> GPDRSFRWKYHQFRFLCHSNALPSHVKISVSRQTLFEDSFQQIMNMKPYDLRRRLYIIMRGEEGLDYGGIAREWFFLLSHEVLNPMYCLFEYAGKNNYCLQINPASSINPDHLTYFRFIGRFIAMALYHGKFIDTGFTLPFYKRMLNKRPTLKDLESIDPEFYNSIVWIKENNLEECGLELYFIQDMEILGKVTTHELKEGGESIRVTEENKEEYIMLLTDWRFTRGVEEQTKAFLDGFNEVAPLEWLRYFDEKELELMLCGMQEIDMSDWQKSTIYRHYTKNSKQIQWFWQVVKEMDNEKRIRLLQFVTGTCRLPVGGFAELIGSNGPQKFCIDKVGKETWLPRSHTCFNRLDLPPYKSYEQLREKLLYAIEETE;> XDPANWECRYAAFNCFIQX

Here, we report a general and rapid method for discovering α-helically constrained (Helicon) polypeptides that cooperatively induce the interaction between two target proteins without relying on previously known binders or an intrinsic affinity between the proteins. We show that Helicons are capable of binding every major class of E3 ubiquitin ligases, which are of great biological and therapeutic interest but remain largely intractable to targeting by small molecules. In addition to possessing increased stability and membrane permeability, Helicons are capable of binding large, flat protein surfaces that are inaccessible to targeting by small molecules, and Helicons have been developed to target a range of PPI targets in cells and in vivo. Characterizing Helicon-E3 co-structures and mechanisms of action, we identified new binding sites for α-helices on the E3 surfaces, as well as potential probes of the disease-linked E3, WWP123,24, highlighting the generality of our approach against this therapeutically important target class.

First, we focused on the NEDD4-like E3 ligases, which make up approximately a third of the HECT family. These include WWP1 and WWP2, which each consist of four tandem WW domains and a catalytic HECT domain at the C-terminus that transfers ubiquitin from a bound E2 first to itself and subsequently to the target substrate. Group 2 Helicons, the pan-HECT group including C73, bind both HECT domains, while Group 3 Helicons, the WWP2-HECT group including C72, bind only the WWP2 HECT domain (WWP2HECT). We next solved the crystal structures of five Helicons, four in complex with WWP2HECT representing all three groups of HECT-binding clusters, and one from Group 1 with WWP1HECT. These structures revealed three distinct Helicon binding sites on WWP2HECT. In all of the structures, we found that the HECT domains adopted similarly closed (inhibited) conformations. The WWP2 proteins in the co-structures with H301, H305, and H308 share a low root-mean-square deviation (RMSD = 0.5–0.8 Å) and are shown overlaid. Consistent with their ability to impact the catalytic activity of WWP2HECT, H301 binds near the E2 interface, while H305 and H308 may restrict the conformational change involved in activating this domain. While the WWP2 linker region is mostly helical, it is linear where it overlaps the H308-binding site.N-{3-[4-(4-phenylthiophen-2-yl)phenyl]propanoyl}-L-alpha-glutamyl-L-alpha-glutamyl-amide | C29 H31 N3 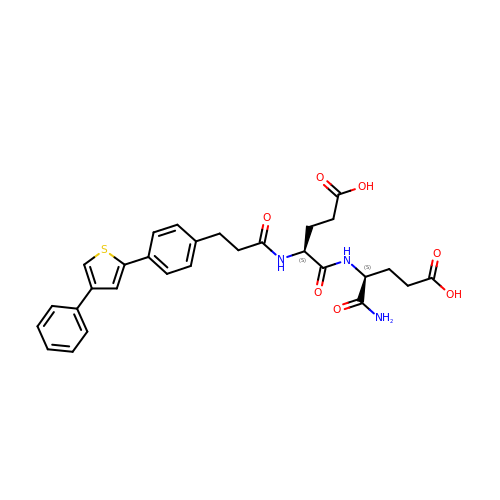O7 S | MMIHYNVQXYWTFM-GOTSBHOMSA-N>MRILVTNDDGIQSKGIIVLAELLSEEHEVFVVAPDKERSATGHSITIHVPLWMKKVFISERVVAYSTTGTPADCVKLAYNVVMDKRVDLIVSGVNRGPNMGMDILHSGTVSGAMEGAMMNIPSIAISSANYESPDFEGAARFLIDFLKEFDFSLLDPFTMLNINVPAGEIKGWRFTRQSRRRWNDYFEERVSPFGEKYYWMMGEVIEDDDRDDVDYKAVREGYV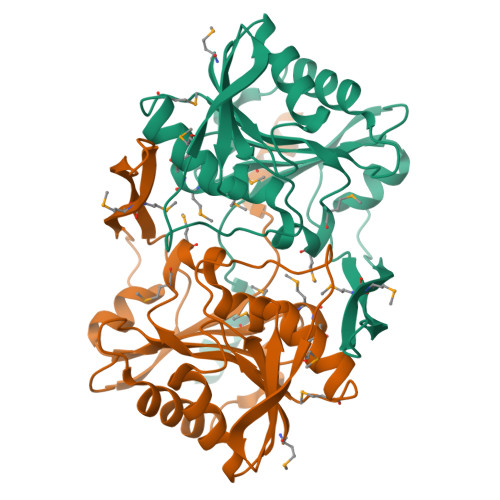SITPIHPFLTNEQCLKKLREVYD[2x]>GPGSMTDRKIPGDRSYTADHEWIDIAPGAATPDGPVRVGITSVAVEALGDLVFVQLPEVGETVSAGESCGEVESTKTVSDLIAPASGQIVEVNTAAVDDPATIATDPYGAGWLYSVQPTAVGELL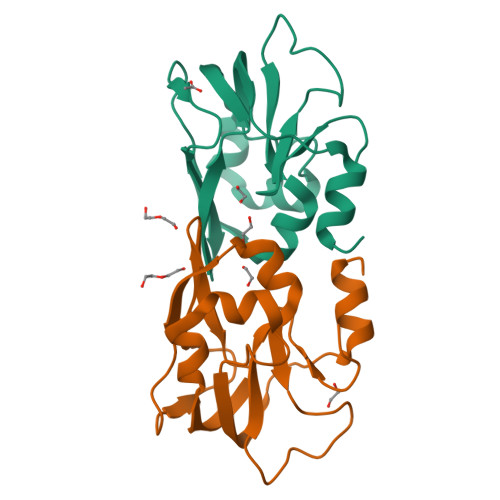TASEYAGQNGLS[4x]1-[3-(thiophen-3-yl)benzyl]piperidin-2-one 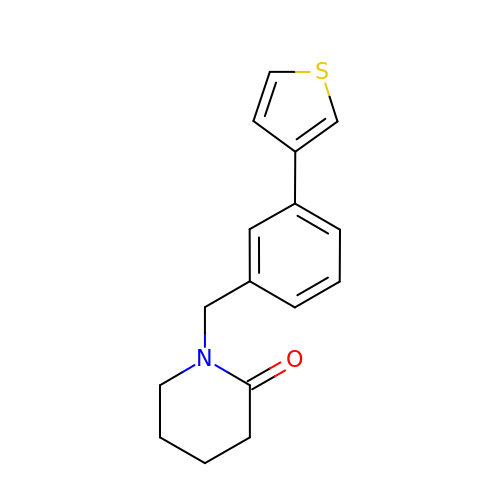| C16 H17 N O S | UMRKGGGHCYSVML-UHFFFAOYSA-N> MRQCVVRRYKMPKNMGVAPRFDTWNEKYEPWEHMKRMGRLVGTGFYIPPEWYNHFRMFPPINHNFQQEKTLNPHNASEPTQDDTSTLSPERVALRDELARKSRLVASEGMR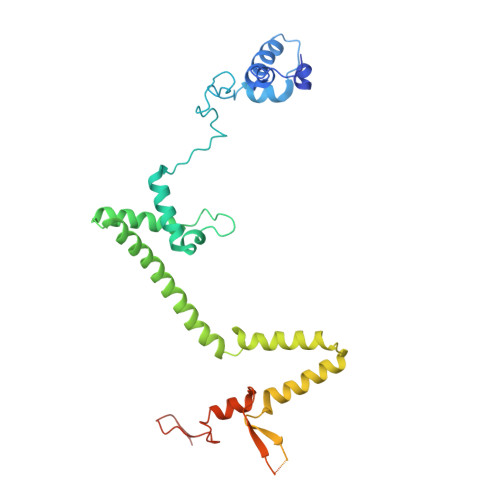YYNIFWVRKPLDTMEKEYYELKRRGVDHGEAIRKVLQGFYSGLAVKKRVAAIQAEEAKLTGRFITMREATVVLGVLAKLHKEQLTPHQVSLLAKEQGETTQSGAKLTAIVSRTQPHVNKEASSPATSEAVGSSTEESLSADALASMLSEDGEQSAVGTRYQVEVKETANDSVRQLREKAEDQTGFPDWYTGESPTYSGTSCSRDGFALMKANK> GSSGSSGMAPWRKADKERHGVAIYNFQGSGAPQLSLQIGDVVRIQ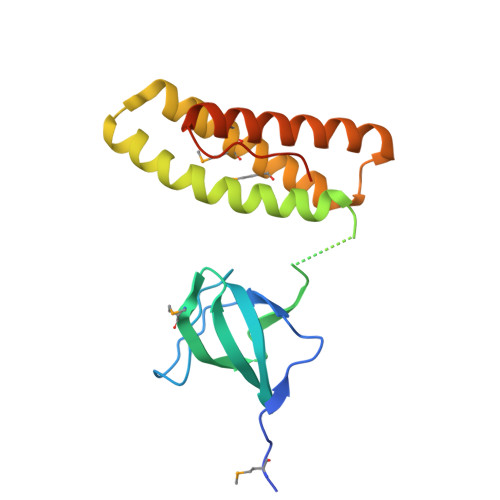ETCGDWYRGYLIKHKMLQGIFPKSFIHIKEVTVEKRRNTENIIPAEIPLAQEVTTTLWEWGSIWKQLYVASKKERFLQVQSMMYDLMEWRSQLLSGTLPKDELKELKQKVTSKIDYGNKILELDLIVRDEDGNILDPDN Diadenosine-5′,5-P1,P4-tetraphosphate (Ap4A) is a ubiquitous second messenger from bacteria to higher eukaryotes, which responds to environmental stresses and cell cycle phases. Ap4A then binds to the histidine triad nucleotide-binding protein 1 (HINT1), thereby disrupting the protein–protein interaction with microphthalmia-associated transcription factor (MITF), and the released MITF eventually promotes the transcription of mast cell activation genes. The HINT1 protein is a compact and symmetric dimer, with two adenosine pockets at opposite sides. Here we report that Ap4A specifically polymerizes HINT1 into (HINT1-Ap4A)n (HAn) filaments in solution and in the activated RBL cells.

HINT1 was reported to efficiently hydrolyze aminoacyl-adenylate (aa-AMP) and ADP, but neither ATP nor ApnA (such as Ap3A, Ap4A, and Ap5A). For comparison, we also solved the HINT1WT-ATP and HINT1WT-Ap5A structures at resolutions of 1.52 and 1.31 Å, respectively. Consistent with previous reports, two HINT1 molecules formed a dimer through the five-stranded β-sheet and the central helix in the crystal structure. Despite having co-crystallized with different ligands, the three structures were nearly identical, with root mean square deviations (RMSDs) < 0.083 Å. However, in all the three structures, only the electron density corresponding to an AMP molecule was observed in the adenosine pocket, indicating that the ligands had been hydrolyzed by the HINT1WT protein during the crystallization, which took 3–7 days at 18 °C with a high protein concentration of ~2 mM.

>[2x]SLMADEIAKAQVARPGGDTIFGKIIRKEIPAKIIFEDDRCLAFHDISPQAPTHFLVIPKKHISQISVAEDDDESLLGHLMIVGKKCAADLGLNKGYRMVVNEGSDGGQSVYHVHLHVLGGRQMHWPPG alpha-D-allofuranose | C6 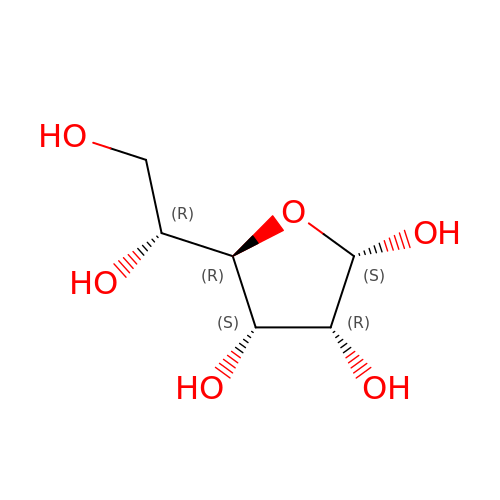H12 O6 | AVVWPBAENSWJCB-RXRWUWDJSA-N> MTKSLFRQSFLFDSLDLDHPMVAQTVRTEQGVTLKLHQRGVLEVIPAQTDAATKNMVISCGIHGDETAPMELLDKWIDDIVSGFQPVAERCLFIMAHPQATVRHVRFIEQNLNRLFDDKPHTPSTELAIADNLKVLLRQFFANTDEHSRWHLDLHCAIRGSKHYSFAVSPKARHPVRSRSLMQFIEQAHIEAVMLSNAPSSTFSWYSAEHYAAQALTLELGQVARLGENLLDRLLAFDLAMRDLISRHKPEHLPRKSVMYRVSRTIVRLHDDFDFRFSDDVENFTAFMHGEVFG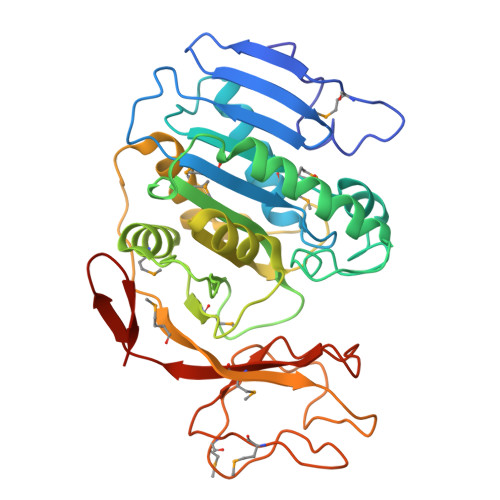HDGDKPLMAKNEGEAIVFPNRKVAIGQRAALMVCKVNTRYEDDQLVYDLEHHHHHH> GPLGHMSIFEKDLMAYFDENLNRNWRGREHWKV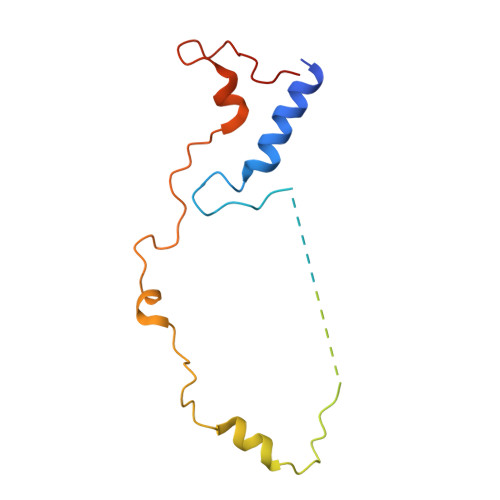RNFKKANLVNKESDLLEETRTTIGDTTDKNTTDDKSMDTKKKHKQKKVLEIDFFKTDDSFEDKVFASKGRTKIDMPIKNRKNDTHYLLPDDFHFSTDRITRLFIKPGQKMSLFSHRKHT>[13x]MRKFILSLSILLSALLVACSSRNHYGDTGSLAGLQAMADSKYTRAQKKQKMGKIREMALKETALSVGAQAGLAWRAKIIDEQLNKQARNLDAIYDFNSLVLEHNILPPVLLEGRNTLNLADAQSIRISDRTYKVAKQAHFITTPPTWRQYLWMDYVKPEAPNVTLLPKTKAEKEIWCIYTERGWKNGIDQANTILEENIARIKEDFGGMILYRKLLAMNMVSPPYVSHTDLGVTGDGSEIHIDDRVLRITALPELNVNSAEWRAAVAKDENALERFKNMEKLANQAKIVITNKSWQPIIAPVS;>MNNNKIVIMFIFSALLAGCAGTMKFKKPPINNPSDDATIKLAEAAVSVSDSMLEMAKVEKVITPPSKDNTLTIPNAYNLQARASVDWSGPIEELTARIAKAAHFRFRVLGKSPSVPVLISISTKDESLAEILRDIDYQAGKKASIHVYPNSQVVELRYAKIYS[26x];>[31x]MMAEHDQNNDEYKFAELDSYDMDQAGESDLDSEASYQSGKEGLTKKKDIKRNALIAIGAVVFIMVMYKIIGWMFFSDKSSQVTSKPAIPPVTQVATPQPVQTIPTTTPIQQVQPTTIIEDDPDLKKKVSAIEMTQQSLRSEVNALSEQINAVNNNIKNLNAQIVNLNQIIGNMSNQIARQSEVINVLMARTTPKKVVKVSRPIVQARIIYYIQAVIPGRAWLIGSNGSTLTVREGSKIPGYGMVKLIDSLQGRILTSSGQVIKFSQEDS;>MASKKENLKSLFSNTRTRVIIIFTAALLIIAVVIGFFKIRGATTGSIAAAEVSTVPGGIQSIPGVLDPTAQYAKLQEEQNITQAQVAEKTGGSAIPTIIRTQALGEGVGVIGSQSGVGFAALAQEELGGPQRSLWIQELQDGSCSKSVITKVVNQGAQLTDLKAACSCVQLKDSGYGLQELEQVCECKELKSAGYNARQLKEAGYSAGRLRNCGFDACELRNAGFTAQEMKDGGFSDGELKGAGFSDAEIAKASGLPDGITADDVRKAGCGAAALAKLRQAGVSASAIRKISGCTAEQLKAAGYTAKELKDAGFSAADLRRAGFSAAELKDAGFTARDLLNAGFTPADLAKAGFSDAQIKAAQAELPPGITPQDVKNAGCDVEALKKEREAGVSAALIRQYAGCSAQALKAAGFTDADLANAGFTPAQISAATPLSDAEIKAAGCDPDKLKKLFSAGVSAKRIKELNGCSAEALKAAGYDAQSLLAAGFTPQELLAAGFTPKQLEDAGLNPVSIIADGRVADCSVESLKKARAAGVSALTIKQTLGCSAAALKAAGYTAKELKDAGFTAAELKAAGFSAKELKDAGFTAKELRDAGFSAQELKDVGFSAKDLKDAGFSAAELKAAGFTAAQLKAAGFSAKDLKDAGFSAAELKAAGFSAKELKDAGFSASDLKNAGFSAKELKDAGFSASDLKSAGFSASELKNAGYSADELKKAGYTSAELRNAGFSPQESAVAGLQGPDLQQLDSSITGIPSIPGATPRPTTSDAASSAEQLQAILQKQNEQLAEQKYQQEIQQRTSDMLTAATQLVQDWKQVETQVYTEGTEETKTSGGESAVPGTGTGTGSNNQPVDQGAVSAQNQAIIKTGDIMFAVLDTSVNSDEPGPILATIVTGKLKGSKLIGSFNLPSNADKMVITFNTMSIPGAEKTISISAYAIDPNTARTALASRTNHHYLMRYGSLFASSFLQGFGNAFQSANTTITIGGTGGGNNITVANGVGRSTLENAVIGLATVGKAWSQQAQQLFNTPTTVEVYSGTGLGILFTQDVTTI[34x];>MMKKYDQLCKYCLVIGLTFSMSCSIYAADQSDDAQQALQQLRMLQQKLSQNPSPDAQSGAGDGGDNAASDSTQQPNQSGQANAPAANQTATAGGDGQIISQDDAEVIDKKAFKDMTRNLYPLNPEQVVKLKQIYETSEYAKAATPGTPPKPTATSQFVNLSPGSTPPVIRLSQGFVSSLVFLDSTGAPWPIAAYDLGDPSSFNIQWDKTSNTLMIQATKLYNYGNLAVRLRGLNTPVMLTLIPGQKAVDYRVDLRVQGYGPNAKSMPTEEGIPPSANDLLLHVLEGVPPPGSRRLVVSGGDARAWLSNEKMYVRTNLTILSPGWLASMTSADGTHAYEMQKSPVLLVSWHGKVMQLKVEGL[18x];>[13x]MRSLRTNYIYVLFKTTGLLFLLLLSACNRSGYIPENEVPKLPCRVDGACDATIIKMMTDLNKKGIKVASVGQNYLISIPASALFADQSPRLNWASYSLLNEIAAFLKQFRKIAITVTSYSSKYVSVKRERALTLARSRVVSEYLWSQGVDSRIIFTQGLGSDKPITSYTLGGDRSPNARVEITFRRAVA;>MRNLMRCLIMIKSLIKGVDMSRKLAKTRILGYGLMICFLAGCFHPPYNNFQPDRRAVKRVGVDTGIGAVAGAIASGTASGTLIGAAAGGTVGLVASIYRDSKRKIIRDLQKQDIQYVEYGDTRTLIIPTDKYFMFSSPRLNEICYPGLNNVIRLLNFYPQSTIYVAGFTDNVGSRSHKRKLSQAQAETMMTFLWANGIAAKRLKAEGYGDKNAISDNAIIHGSAQNRRIEIQWFTSPAQPPQPQMAYVK[13x];>[13x]MLKRCYLLILLMFVLASCAHHKPQTPPAEVKKQGTSSTRQFRQVSSFNQIVVQGRLNVNLHTGYNKPEVMLRGDPRDLVQVRTIVKQNTLYVSLGQGYPDYGAVTVDIKTKFLNRFRYEGAGVVTGNNLRTSYLDLYLANEGTTRLAGNIGLQKLEAVGNGVTQINGVSSRNLQIVLKGDPKVLISGFVNLRQLDMYGKGTLSLYWIKSDTLTIRAKKAAKIQLAGIVNRLDVELWDFAQFKGKYLRAQRSFVKTHDKSVAEISAVNHQSSLATDASDIYYYNLSKTRADFMAFNGSVLDMREWGQSDLKDFDRYNKQFP;>MLFLKIKTNQRTTMNILKPKAFLLASVFVLSISPAFAADGCCSKMGGINYCDSSAGRLVCNNGFYSTCYCTRHAVMDLQFLMGCCLWHGGVYPQLNSSGLVVCNDGYVSEECSLQKPVEQISVY[13x]

Legionella pneumophila is an opportunistic pathogen that causes the potentially fatal pneumonia known as Legionnaires’ disease. The pathology associated with infection depends on bacterial delivery of effector proteins into the host via the membrane spanning Dot/Icm type IV secretion system (T4SS). The Dot/Icm complex of L. pneumophila is one of the largest known T4SSs. The Dot/Icm T4SS has as many as 300 protein substrates, a striking contrast to the H. pylori Cag and B. pertussis Ptl T4SSs, each of which transports only one virulence factor.

Using 3D variability analysis, we reconstructed a total of five maps that displayed differences in the way the outer membrane cap (OMC) and periplasmic ring (PR) were positioned. These maps led to the identification of an approximate 16-fold symmetry about the center of the dome positioned within the OMC. Within this dome there are 16 α-helices that appear nearly identical at this resolution. Indeed, a model of the C-terminal domain of DotG generated in Swiss Model using VirB10 as a template fits into the resolved dome density (Waterhouse et al., 2018). However, we have unexpectedly uncovered that the Dot/Icm incorporates only 16 copies of DotG into the OMC dome out of the 18 DotG copies in the PR, giving rise to another symmetry mismatch within this system. Based on the structure of DotG modeled within the PR (residues 791–824) and the homology model fit into the dome density (consisting approximately of residues 857–1046), we hypothesize that DotG extends from the PR to the dome, though a physical connection between the two structures is not observed. (A) Two DotC were observed in the maps that were reconstructed during 3D variability analysis, one which contains an N-terminal extension (DotCLong) and one which does not (DotCshort). In contrast, the N-terminal extension of DotC was modeled as two relatively large helices positioned near DotG and bridging adjacent asymmetric units. Notably, this portion of DotC was only observed in either four or five of the 13 copies of DotC observed in each map. The movie shows that the OMC dome, OMC disk, and PR of Dot/Icm T4SS can accommodate various orientations in relation to each other that suggest that the complex could undergo a ratcheting motion, in which the dome and PR rotate back and forth about the central axis with the different regions of the complex tethered together by the physical connections across the symmetry mismatches.>[5x]MHHHHHHGSDDDDKRPEAKSAQPADGWKGERPRSEEDNELNLPNLAAAYSSILSSLGENPQRQGLLKTPWRAASAMQFFTKGYQETISDVLNDAIFDEDHDEMVIVKDIDMFSMCEHHLVPFVGKVHIGYLPNKQVLGLSKLARIVEIYSRRLQVQERLTKQIAVAITEALRPAGVGVVVEATHMCMVMRGVQKMNSKTVTSTMLGVFREDPKTREEFLTLIRS

Guanosine triphosphate (GTP) cyclohydrolase I (GCH1) (EC:3.5.4.16) catalyzes the conversion of GTP to dihydroneopterin triphosphate (H2NTP). This reaction is the first and rate-limiting step involved in the de novo synthesis of tetrahydrobiopterin (BH4). The effects of GFRP on GCH1 occur via formation of heteromeric protein complexes between GCH1 and GFRP, which are dependent on the intracellular concentrations of the effector molecules phenylalanine or BH4. GCH1−GFRP complexes consist of one GCH1 decamer flanked by two pentameric GFRP complexes.

AXSP0056BS (cpd-1) was identified as an allosteric GCH1 inhibitor in an enzymatic assay with half maximal inhibitory concentration (IC50) values of 4 µM. From one cocrystallization campaign, surprisingly, we obtained two independent structures of allosterically inhibited GCH1: one fully inhibited form (xtal_GCH1_allosteric) with all allosteric sites occupied by inhibitor, and a partially inhibited form (xtal_GCH1_allosteric), in which only two of five allosteric pockets in each GCH1 pentamer were occupied with cpd-1. Cpd-1 binds to two allosteric sites of each GCH1 pentamer, which are located in the interface of chains A and B and of chains D and E. The three remaining allosteric sites per pentamer remain unoccupied. Binding of inhibitors into the allosteric site, which is flanked by two distinct protomers, trigger different process changes in the respective subunits. Interactions of residues of one subunit (chains A or D, right) trigger conformational rearrangements of the respective subunit, while the conformation of the other subunit (chains B and E, left) does not change. Binding of cpd-1 induces concomitant approximation of the C-terminal helices and β-strands of subunits A and B (D and E, respectively), while distances between helices B and D, C and D, and A and E remain unchanged relative to the active state of the enzyme. Analysis of the conformational states of all protomers show that chains A and D exhibit an inhibitory xtal_GCH1+allosteric-like state, while protomers B, C, and E are in an apo-like conformation in terms of helix bundle and β-barrel positioning and curvature. Region A is ordered in protomers A, C, and D, but is highly flexible in chains B and E. This observation agrees with the also drastically increased flexibility of region A in the remaining allosteric ligand-bound EM and X-ray structures.> ATFISVQLKKTSEVDLAKPLVKFIQQTYPSGGEEQAQYCRAAEELSKLRRAAVGRPLDKHEGALETLLRYYDQICSIEPKFPFSENQICLTFTWKDAFDKGSLFGGSVKLALASLGYEKSCVLFNCAALASQIAAEQNLDNDEGLKIAAKHYQFASGAFLHIKETVLSALSREPTVDISPDTVGTLSLIMLAQAQEVFFLKATRDKMKDAIIAKLANQAADYFGDAFKQCQYKDTLPKEVFPVLAAKHCIMQANAEYHQSILAKQQYYFGEEIARLQHAAELIKTVASRYDEYVNVKDFSDKINRALAAAKKDNDFIYHDRVPDLKDLDPIGKATLVKSTPVNVPISQKFTDLFEKMVPVSVQQSLAAYNQRKADLVNRSIAQMREATTLANGVLASLNLPAAIEDVSGDTVPQSILTKSRSVIEQGGIQTVDQLIKELPELLQRNREILDESLRLLDEEEATDNDLRAKFKERWQRTPSNELYKPLRAEGTNFRTVLDKAVQADGQVKECYQSHRDTIVLLCKPEPELNAAIPSANPAKTMQGSEVVNVLKSLLSNLDEVKKEREGLENDLKSVNFDMTSKFLTALAQDGV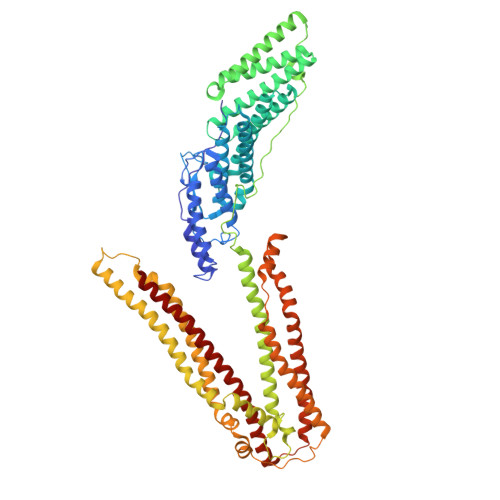INEEALSVTELDRVYGGLTTKVQESLKKQEGLLKNIQVSHQEFSKMKQSNNEANLREEVLKNLATAYDNFVELVANLKEGTKFYNELTEILVRFQNKCSDIVFAR> MDTNDNAPKFERPSYEAELSENSPIGHSVIQVKANDSDQGANAEIEYTFHQAPEVVRRLLRLDRNTGLITVQGPVDREDLSTLRFSVLAKDRGTNPKSARAQVVVTVKDMNDNAPTIEIRGIGLVTHQDGMANISEDVAEETAVALVQVSDRDEGENAAVTCVVAGDVPFQLRQASETGSDSKKKYFLQTTTPLDYEKVKDYTIEIVAVDSGNPPLSSTNSLKVQVVDVNDNALEHHHHHH

Protocadherin-1 (PCDH1) is a non-clustered δ1 protocadherin involved in respiratory diseases. PCDH1 has seven EC repeats (labeled EC1 to EC7 from N to C-terminus), a single pass transmembrane domain and a cytoplasmic domain with the three conserved motifs (CM1–CM3) typical of the δ1 subgroup. PCDH1 may bind bronchial epithelial cells and epithelial cells of the airway mucosa together by mediating homophilic adhesion and helping in forming the epithelial barrier. Here we use bead aggregation assays to show that repeats EC1 to EC4 form the minimal adhesive unit for human (Homo sapiens [hs]) PCDH1, despite its longer extracellular domain with seven EC repeats.

The first two, PCDH1 EC3-4bc at 3.05 Å and PCDH1 EC1-4bc at 2.85 Å, were obtained using bacterially produced protein. The PCDH1 EC3-4bc structure (T216 to Q438) had one molecule in the asymmetric unit, had poor density for three loops in EC4 that were not modeled, and it was used as an initial model for phasing the PCDH1 EC1-4bc structure by molecular replacement. The RMSD for the shared Cα atoms among the chains of PCDH1 EC1-4bc and PCDH1 EC3-4bc was also low (~1.5 Å). Crystal contacts in the PCDH1 EC3-4bc structure are not expected to reveal a physiologically relevant interface as their areas are small and repeat EC1, required for trans binding, is absent. Nevertheless, some of these contacts could represent low-affinity transient intermediates for both trans and cis (from the same cell) interactions.>[2x]NADNYKNVINRTGAPQYMKDYDYDDHQRFNPFFDLGAWHGHLLPDGP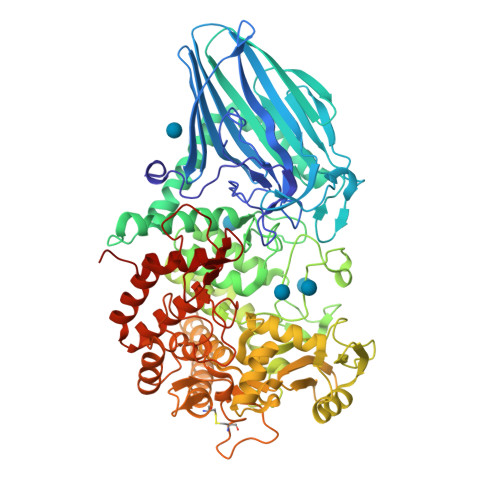NTMGGFPGVALLTEEYINFMASNFDRLTVWQDGKKVDFTLEAYSIPGALVQKLTAKDVQVEMTLRFATPRTSLLETKITSNKPLDLVWDGELLEKLEAKEGKPLSDKTIAGEYPDYQRKISATRDGLKVTFGKVRATWDLLTSGESEYQVHKSLPVQTEINGNRFTSKAHINGSTTLYTTYSHLLTAQEVSKEQMQIRDILARPAFYLTASQQRWEEYLKKGLTNPDATPEQTRVAVKAIETLNGNWRSPGGAVKFNTVTPSVTGRWFSGNQTWPWDTWKQAFAMAHFNPDIAKENIRAVFSWQIQPGDSVRPQDVGFVPDLIAWNLSPERGGDGGNWNERNTKPSLAAWSVMEVYNVTQDKTWVAEMYPKLVAYHDWWLRNRDHNGNGVPEYGATRDKAHNTESGEMLFTVKKGDKEETQSGLNNYARVVEKGQYDSLEIPAQVAASWESGRDDAAVFGFIDKEQLDKYVANGGKRSDWTVKFAENRSQDGTLLGYSLLQESVDQASYMYSDNHYLAEMATILGKPEEAKRYRQLAQQLADYINTCMFDPTTQFYYDVRIEDKPLANGCAGKPIVERGKGPEGWSPLFNGAATQANADAVVKVMLDPKEFNTFVPLGTAALTNPAFGADIYWRGRVWVDQFWFGLKGMERYGYRDDALKLADTFFRHAKGLTADGPIQENYNPLTGAQQGAPNFSWSAAHLYMLYNDFFRKQ>[2x]QTSGPMSLESLAPPESTDEGAETESPEPGDEGEPGRSGLELEPEEPPGWRELVPPDTLHSLPKSQVKRQEVISELLVTEAAHVRMLRVLHDLFFQPMAECLFFPLEELQNIFPSLDELIEVHSLFLDRLMKRRQESGYLIEEIGDVLLARFDGAEGSWFQKISSRFCSRQSFALEQLKAKQRKDPRFCAFVQEAESRPRCRRLQLKDMIPTEMQRLTKYPLLL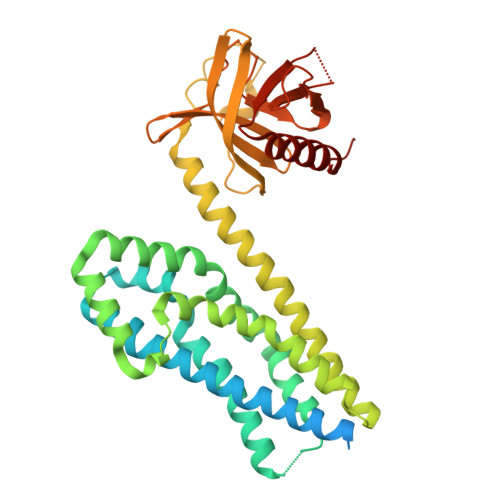QSIGQNTEEPTEREKVELAAECCREILHHVNQAVRDMEDLLRLKDYQRRLDLSHLRQSSDPMLSEFKNLDITKKKLVHEGPLTWRVTKDKAVEVHVLLLDDLLLLLQRQDERLLLKSHSRTLTPTPDGKTMLRPVLRLTSAMTREVATDHKAFYVLFTWDQEAQIYELVAQTVSERKNWCALITETAGSLKVPA> GHMAAPARFCVYYDGHLPATRVLLMYVRIGTTATITARGHEFEVE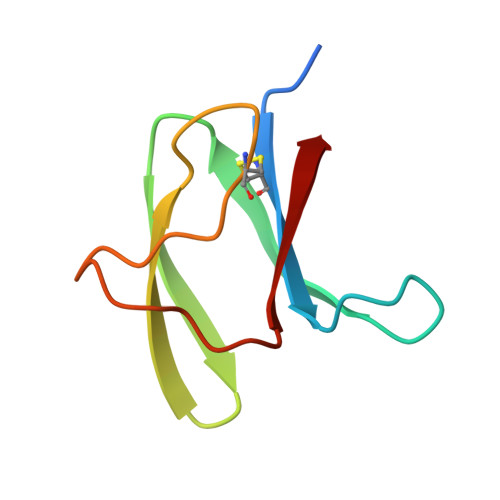AKDQNCKVILTNGKQAPDWLAAEPY> DNIEDIPLGSSEQDPYDFFTLSDRNVMNSDMKKNIVQWNSRYSYNQLKNKDSLIMFLVEIFRSLFVSNCIDKNIDNVLLSIEEMFIDHYYNPQHSRLKYLIDDVGIFFTKLPITKAFHTYNKKYRITKRLYAPPTFNEVRHILNLAQILSLEEGLDLLTFDADETLYPDGHDFNDEVLASYISCLLKKMNIAIVTAASYNNDAEKYQKRLENLLKYFSKHNIKDGSYKNFYVMGGESNYLFKCNEEATLYSVPENEWRHYKKFVDYDTVQEILNISEKCLEKVIKDFGLCAQIQRKEKSIGLVPNKIPSLNIKNEQKNYMIKYEVLEEAVIRIKKEII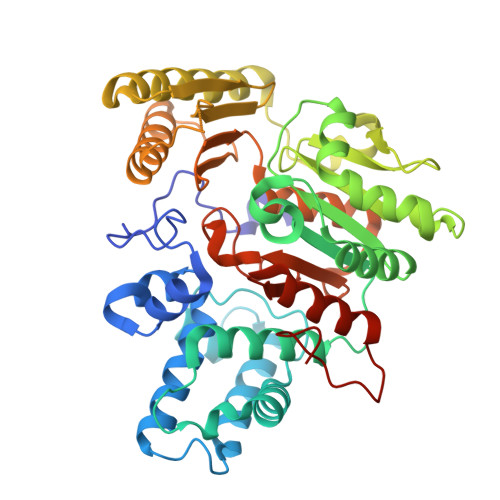KNKITAPYCAFNGGQDLWVDVGNKAEGLLILQKLLKIQKKKCCHIGDQFLHSGNDFPTRFCSLTLWVSNPQETKACLKSIMHLNIKSFIPEVLYENQ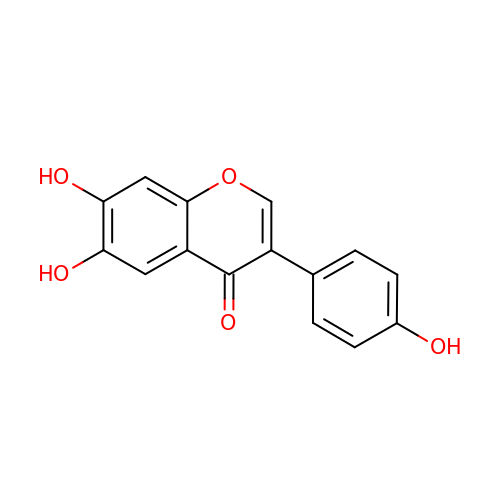6,7-dihydroxy-3-(4-hydroxyphenyl)-4H-chromen-4-one | C15 H10 O5 | GYLUFQJZYAJQDI-UHFFFAOYSA-N N-[2-{4-[(2S)-4-(methylsulfonyl)morpholin-2-yl]-1,3-thiazol-2-yl}-4-(morpholin-4-yl)phenyl]-1H-imidazole-2-carboxamide | 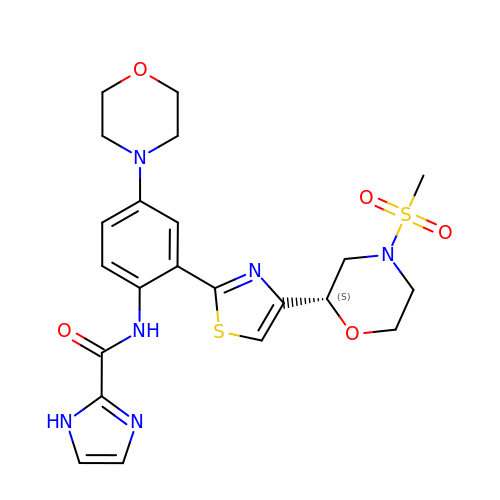C22 H26 N6 O5 S2 | WWTNLDQWEKRXNB-IBGZPJMESA-N> GDEDYPKSHIEPYDTELLSIKILNAGANGDKVVEGTIDEAKKTINFPRLDVETDFSALSIEAELSEGAALQSEVMDYSMDAETNEKTQVLRIINHNRYKDYLMKVRKRVPVFGADFEKPTVYNFSGDNIYSDFATNYTRCASYDGEHVLVVSRPTTPNFHTPHLLKVSDLKRGEIKPIMLDVTGVKGGTYDYNMGALINGHVYLSSLSGGKVSPFKIYYWETPTSNPEVIANINVGNIPGAGNRHGDNASYNIDENGNGFIFFGDNAATEFLKVPISGHKTVDIGNIKVLPSKSDATMVTNVYRVGDTDQYLWSGIRVPVTLVDESLGEKYKSKIAGEAVAPKVVTFNEERYLLVCTAGQGAASKASIALEVYDLTKGETIEDALKKFDEGENHNPIYQFKLGGSGNGNALA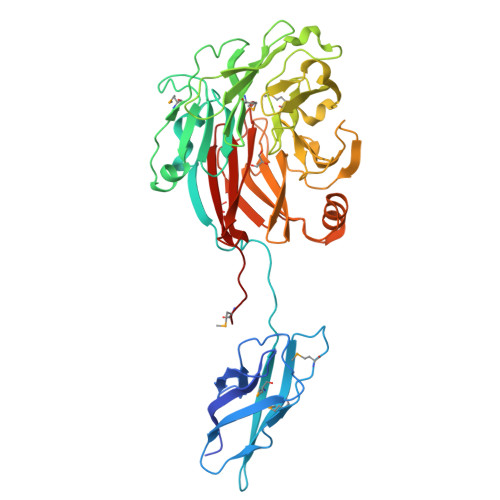QTDYYIEKDENGKDAKLCLFASRTQSGFVICEFPIKQEEMD>[4x]MNRSALDFRHFVDHLRRQGDLVDVHTEVDANLEIGAITRRVYERRAPAPLFHNIRDSLPGARVLGAPAGLRADRARAHSRLALHFGLPEHSGPRDIVAMLRAAMRAEPIAPRRLERGPVQENVWLGEQVDLTRFPVPLLHEQDGGRYFGTYGFHVVQTPDGSWDSWSVGRLMLVDRNTLAGPTIPTQHIGIIREQWRRLGKPTPWAMALGAPPAALAAAGMPLPEGVSEAGYVGALVGEPVEVVRTQTNGLWVPANTEIVLEGEISLDETALEGPMGEYHGYSFPIGKPQPLFHVHALSFRDQPILPICVAGTPPEENHTIWGTMISAQLLDVAQNAGLPVDMVWCSYEAATCWAVLSIDVQRLAALGTDAAAFAARVAETVFGSHAGHLVPKLILVGNDIDVTEIDQVVWALATRAHPLHDHFAFPQIRDFPMVPYLDAEDKARGSGGRLVINCLYPEQFAGQMRAATASFRHAYPTALRRRVEERWSDYGFGDA

The UbiD family of reversible (de)carboxylases depends on the recently discovered prenylated-FMN (prFMN) cofactor for activity. Here, we show that the Pseudomonas aeruginosa virulence attenuation factor PA0254/HudA is a pyrrole-2-carboxylic acid decarboxylase. We here report that the UbiD-like Pseudomonas aeruginosa virulence attenuation factor PA0254/HudA is a close homologue of Bacillus megaterium PYR2910 pyrrole-2-carboxylate (P2C) decarboxylase and show that PA0254 is capable of prFMN-dependent decarboxylation of P2C as well as carboxylation of pyrrole. Substrate screening reveals HudA and selected active site variants can accept a modest range of heteroaromatic compounds, including thiophene-2-carboxylic acid. Together with computational studies, our data suggests prFMN covalent catalysis occurs via electrophilic aromatic substitution and links HudA activity with the inhibitory effects of pyrrole-2-carboxylic acid on P. aeruginosa quorum sensing.

Crystals obtained in the presence of 100 mM imidazole (acting as the buffering agent) did occasionally yield nontwinned crystals which were used for data collection and refinement. A structure was obtained to 1.65 Å resolution using the apo-PA0254 structure as a molecular replacement model. The asymmetric unit (AU) contains two PA0254UbiX dimers, with each monomer found to bind a prFMN cofactor via Mn2+ and K+ coordination. The overall conformation and position of the prFMN binding domain is highly similar in the four monomers present in the AU and resembles the closed conformation previously observed for the A. niger Fdc1. In each of the four monomers, additional electron density was observed located above the prFMN cofactor. The density was modeled as an imidazole derived from the crystal mother liquor. In two of the PA0254UbiX monomers, the imidazole density was continuous with the prFMN density, suggesting a covalent bond between the imidazole C2 and the C1′ of the prenyl-derived prFMN ring. The electron density in the other two monomers was noncontinuous between the imidazole and prFMN and thus modeled as a noncovalent, stacking interaction between imidazole and the prFMN aromatic plane. In both the covalent and the noncovalent ligand complexes, the imidazole N1 is within the hydrogen-bonding distance of the N318 amide side chain. Hydrophobic interactions with Y279, W322, F432, and M434 largely occlude the imidazole from the solvent, with the exception of the water molecule hydrogen bonding to the imidazole N3.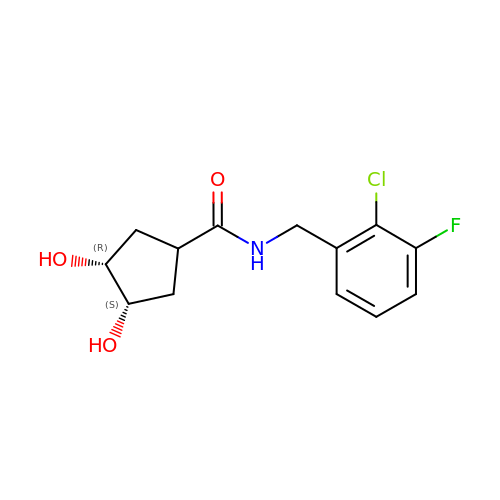Optactamide | C13 H15 Cl F N O3 | NDBRBNVUHSZFIV-GUDFOSOFSA-N>[2x]SNAMEGNMLYHRYLKPNSEYYKKIEVRGKDNIYELNDIPDTYAVFLDNESVWKHYHVKGSTLPEQGWKIHVTSSLEDSKDVLDKVARLCIDKKIEFKHLKDKDSFMKMNSKNANRASSGKFITIYPTNNEVFVELLEMISLAIQDFKKGPYILNDKRWKNSNVFYRYGGFKGIFNEHGEHCIRDKEGNLIKDQRNPFYQVPDFVKDFDDYLNTINNSGELENKGESRLGKYKIETALSFSNAGGVYLATRKKDNLKVIIKEARPSAGLDGAAQDALARQKIEYDALKKLKDVSGVVNLIEYFQEWEHYFLVEEFIEGRDLRQWIAQEFPFFEDNNGMSNHIKDVKMILLQLLDLIDSMHNQGVAMGDLQPANIMVTEDLTVRIIDFETAMPVNSDDRPAMLTTGFVSHEMKVSGARDWFGFKRLVRYLALPVLTSEDLEGYLQYNHLNWIKENYGYEFYSFIVDLQEKCDKRIKDYQTFIPKEINLNDQTSDFNLTSIINKLIIGVESSLTNDERFINGDIRQFEMNGGKFNFLTGGSGAAFTLTKNKSSIAEVDKWIQSVLLDNLPLIEEDGLFTGKTGILALLYDKGYKEVVLNELKILKDNINQTDISIRSGLSGIGLFVISLYLETENKEYLKLAKDLERMIKLNRAKDKQLKVKDWMAVDIGVIDGLSGVSLFYSALYSVTQNQKYLEEAEVLIKEDLESTKKDDVTGVLQTVDNKNRLLPYLSGGSIGVAISIWFLNHVSGQDLYREEMNSILKLSKTRCTISGGLFDGAGSFLLIPSMVKNDKNREVILNEVLNLLNIFLIEKNSYYVYPGQFSYRLADDVYTGSSGIILALMGVIKGNPLYWLPLVNSDEFLARTKVKDLSVTSGKI

In bacteria, Ser/Thr protein kinase-like sequences are found as part of large multidomain polypeptides that biosynthesize lanthipeptides, a class of natural products distinguished by the presence of thioether cross-links. The kinase domain phosphorylates Ser or Thr residues in the peptide substrates. Subsequent β-elimination by a lyase domain yields electrophilic dehydroamino acids, which can undergo cyclase domain-catalyzed cyclization to yield conformationally restricted, bioactive compounds. We also describe the first crystal structures of a class III lanthipeptide synthetase, consisting of the lyase, kinase, and cyclase domains, in various states including complexes with its leader peptide and nucleotide.

To compare the consequences of leader peptide binding on the structure of ThurKC, we carried out numerous attempts to produce the enzyme in the absence of the leader peptide, with no success. Expression of ThurKC in the absence of the leader peptide resulted in an impure protein that was prone to aggregation. Eventually, we were able to grow crystals of ThurKC that were purified with the leader but with most of the peptide removed during purification. The resultant 2.52 Å resolution structure does not show any density for the leader peptide at the binding site but may contain trace amounts that remained throughout the purification process. The structure of this “leaderless” ThurKC shows density for the activation segment and catalytic loops in conformations similar to that observed in the structure of LP-(GS)7-ThurKC. However, a comparison of the respective C-lobes of the two structures reveals that the N-lobe of “leaderless” ThurKC is shifted away from the C-lobe. This movement opens the ATP and peptide-binding sites that are sandwiched between the two lobes. Although there are no changes in the orientation of secondary structural elements that define the activated conformation, the relative movement of the N- and C-lobes in the absence of the leader peptide shifts active site residues too far away to productively interact with ATP and presumably the peptide substrate. The displacement of the N- and C-lobes results in significant movements of both the lyase domain and the cyclase domain. Many of the residues that stabilize interactions between the three domains are displaced and incapable for interaction in the “leaderless” ThurKC structure.The impenetrable nature of the outer membrane is due to the presence of a large, amphipathic glycolipid called lipopolysaccharide (LPS) in its outer leaflet. Assembly of the outer membrane requires transport of LPS across a protein bridge that spans from the cytoplasmic membrane to the cell surface. Here, using structural, biochemical and genetic approaches, we show that these antibiotics trap a substrate-bound conformation of the LPS transporter that stalls this machine. The inhibitors accomplish this by recognizing a composite binding site made up of both the Lpt transporter and its LPS substrate.

We first solved a structure of LptB2FG in the presence of LPS and compound 1 to 3.0 Å resolution. Unexpectedly, compound 1 was found to form extensive contacts with both LptB2FG and a bound LPS molecule, which is a unique mode of inhibition. Because LptB2FG was heterologously expressed in Escherichia coli, the structure we obtained contained copurified E. coli LPS. The compound binding pocket is lined by side chains of several amino acids in the transmembrane (TM) helices of LptF (Glu58, Glu249, Trp271, Val314, Ile317, Arg320 and Thr321) and LptG (Leu36). The ternary complex structure also showed an extensive interface between LPS and 1. The LptB2FG–LPS–1 structure revealed that 1 protrudes into the gate formed between helix 5 of LptF and helix 1 of LptG, suggesting that its binding competes with the LptC TM helix for binding to the complex. The LptB2FG–LPS–1 structure suggested that 1 traps an intermediate state of the LPS-bound Lpt transporter. The drug pose observed in the ternary structures of A. baylyi LptB2FG in complex with E. coli LPS fully explained the resistance mutations that were isolated in Acinetobacter, indicating that contacts with LptFG are critical for drug recognition.

>[2x]MHHHHHHHMEQIAQQQPQTLCIKHLAKNYSKRWVVKDVSFEMQSGQIVGLLGPNGAGKTTSFYMVVGLVRMDKGEIHLDNLDLSDLAMHERARKGIGYLPQEASIFRKLTIAENIMAILETRKDLNKQQRQQRLQELLNDFKITHIKDSLGMSVSGGERRRAEIARALAADPKFMLLDEPFAGVDPISVGDIKDIIRNLKDRGIGVLITDHNVRETLAICEHAYIVSEGAVIAEGSPQDILENEQVRKVYLGDDFTV;> MIIRRYLVKQVVSTSLVVIALLTLIMMGGRLIKYFGVAAQGRLDAGVLFSIIGYRMPEFLTLILPLGFFIGLMLVFGRLYVDHEMAVLNGSGISRIRLGQLLIPLALVFLVIQGILMLWMTPWGLRQFDQLSSSQAVRTGFDLVRPKEFISSGPYTIYAGDLSEDRKNLKDIFFYQRAQKEGKPDVMILAKEATRVVMENETANVVDLIQGRRYEIYPGKAKYSQAEFQRYRLRLENDKSATFETDKVEALPSSKLWNKWNDPVIASEMGWRVFGPFTIVIALMMAVALCEVSPRQGRYYRLIPAIFIFASLIVLLIAIRTRISRDELGVWAYPAALAVYGIAAALFSRKQKLAPKIKKQIKRVRA;> MLARRIVAKHVTKTTALAMLGTTIVLVILQVLFTYLGELSNLKADYSAWQAFLYVLWGAPRYLYEILPISALIGAILGLGTLASNSELIVMRSVGISLWRIVGWVIRSALVLVLLSFALSEWVVPYTNERANSVKSHQSVAALGEVRGYWSREGQRFIYVDYANSQGQLKRIQVVDFDDNYRLKSVTNAEQGQFVKDGQWLLNHSQQMAIQGQGDAVLANAAKQPFSLALQPKYVHMVTIDPEDLSFSQLVSFMNYMREYSQVPKTYQLAFWKKVASPFALITLVLVACSFIFGPLRQQSMGFRLVIALFIGLGFYYLQDFLGYASLVYNPSPAWFVLGPIVLMFVAGSYLLYRAR>[2x]GSRDRMMKLSLIKVVNGCRLGKIQNLGKAGDCTVDIPGCLLYTRTGSAPHLTHQTLRNIHGVPGIAQLTLSSLAEHHEVLAEYKKGVGSFIGMPESLFYCSLHDPVTPGPAGYVTSKSVSVWGFGGR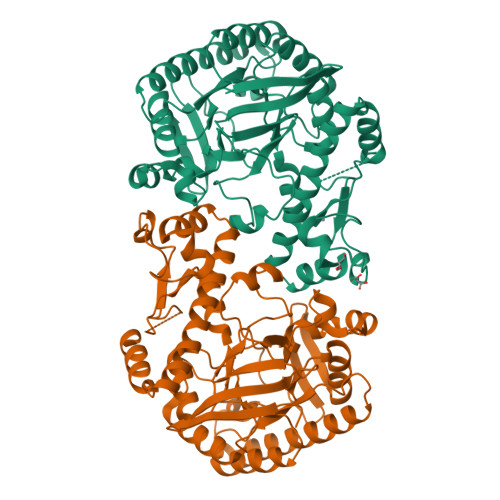VEMTVSKFMAIQEALQPDWFQCLSDGEASCAETTSIKRARKSVDRSLLFLDSCLRLQEESEVLQKSVIIGVIEGGDVMEERLRSARETAKRPVGGFLLDGFQGDPAVTETRLHLLSSVTAELPEDKPRLICGVSRPDEVLECIERGVDLFESFFPYQVTERGCALTFTFDCQLNPEETLLQQNGIQEKIKGLDQAKKIEATGCNQEMTSFEINLKEKKYQEDFDPLVRGCSCYCCKNHTRAYIHHLLMTNELLAGVLLMMHNFEHYFGFFCSIREALKNDTLAQLKELICRQMFGL> MVPISPIETVPVKLKPGMDGPKVKQWPLTEEKIKALVEICTEMEKEGKISKIGPENPYNTPVFAIKKKDST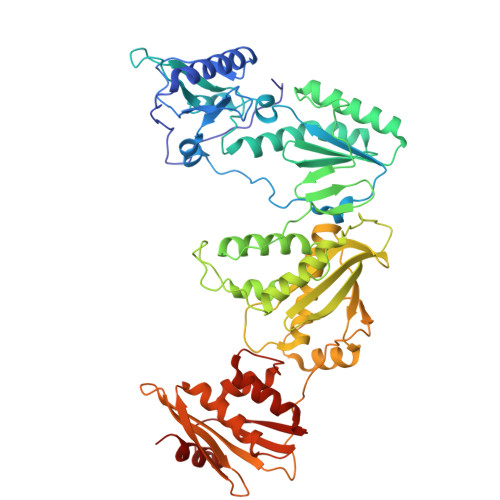KWRKLVDFRELNKRTQDFWEVQLGIPHPAGLKKKKSVTVLDVGDAYFSVPLDEDFRKYTAFTIPSINNETPGIRYQYNVLPQGWKGSPAIFQSSMTKILEPFAAQNPDIVIYQYMDDLYVGSDLEIGQHRTKIEELRQHLLRWGLTTPDKKHQKEPPFLWMGYELHPDKWTVQPIVLPEKDSWTVNDIQKLVGKLNWASQIYPGIKVRQLSKLLRGTKALTEVIPLTEEAELELAENREILKEPVHGVYYDPSKDLIAEIQKQGQGQWTYQIYQEPFKNLKTGKYARMRGAHTNDVKQLTEAVQKITTESIVIWGKTPKFKLPIQKETWETWWTEYWQATWIPEWEFVNTPPLVKLWYQLEKEPIVGAETFYVDGAANRETKLGKAGYVTNKGRQKVVPLTNTTNQKTELQAIYLALQDSGLEVNIVTDSQYALGIIQAQPDKSESELVNQIIEQLIKKEKVYLAWVPAHKGIGGNEQVDKLVSA>VDPTHFEKRFLKRIRDLGEGHFGKVELCRYDPEGDNTGEQVAVKSLKPESGGNHIADLKKEIEILRNLYHENIVKYKGICTEDGGNGIKLIMEFLPSGSLKEYLPKNKNKINLKQQLKYAVQICKGMDYLGSRQYVHRDLAARNVLVESEHQVKIGDFGLTKAIETDKEYYTVKDDRDSPVFWYAPECLMQSKFYIASDVWSFGVTLHELLTYCDSDSSPMALFLKMIGPTHGQMTVTRLVNTLKEGKRLPCPPNCPDEVYQLMR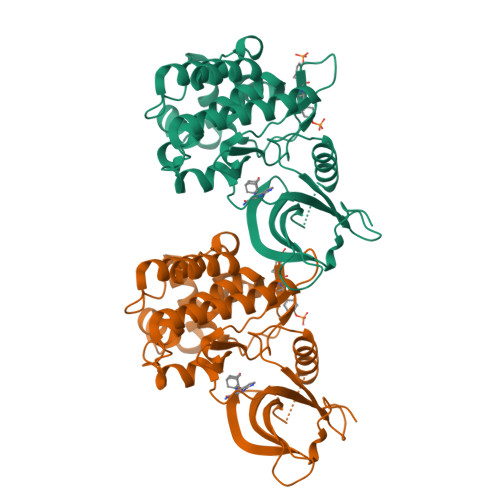KCWEFQPSNRTSFQNLIEGFEALLK[2x]> GPAFEFAVAMMKRNSSTVKTEYGEFTMLGIYDRWAVLPRHSKPGPTILMNDQEVGVLDAKELVDKDGTNLELTLLKLNRNEKFRDIRGFLAKEEVEVNEAVLAINTSKFPNMYIPVGQVTEYGFLNLSGKPTKRMLMYNFPTKAGQCGGVLMSTGKVLGIHIGGNGRQGFS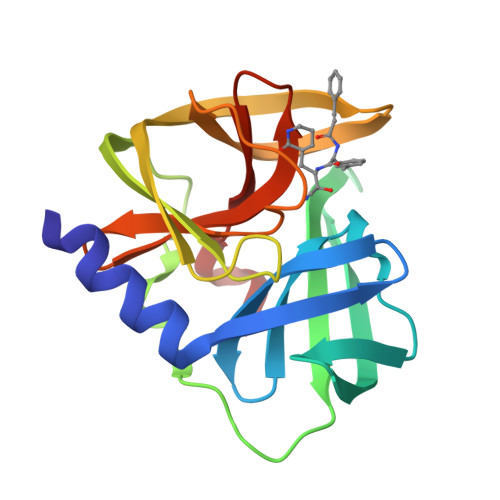AALLKHYFN>[8x]MGQGQWIAARDLSITWV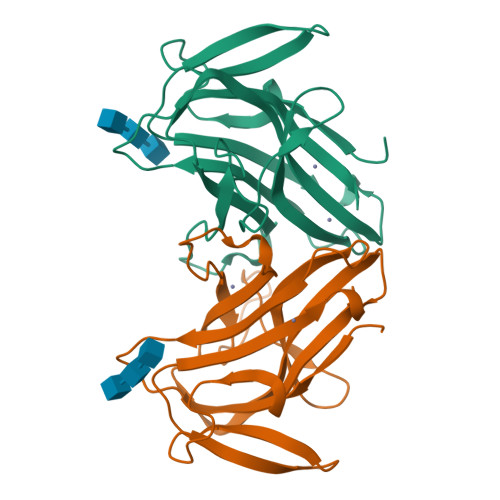DNPQYWTWKTVDPNIEVAELRRVAWLDIYGKIETKNLIRKTSYAVYLVFKLTDNPRELERATASLRFVNEVAEGAGIEGTTVFISKKKKLPGELGRFPHLRSDGWLEIKLGEFFNNLGEDGEVEMRLMEINDKTWKSGIIVKGFDIRPN>[4x]MQRVVVAIVAKRVDGEFMVFTHSGKKNTGILLRDWVVEVEKRGAGEILLTSIDRVGTKSGYDTEMIRFVRPLTTLPIIASGGAGKMEHFLEAFLAGADKVSINTAAVENPSLITQIAQTFGSQAVVVAIVAKRVDGEFMVFTHSGKKNTGIL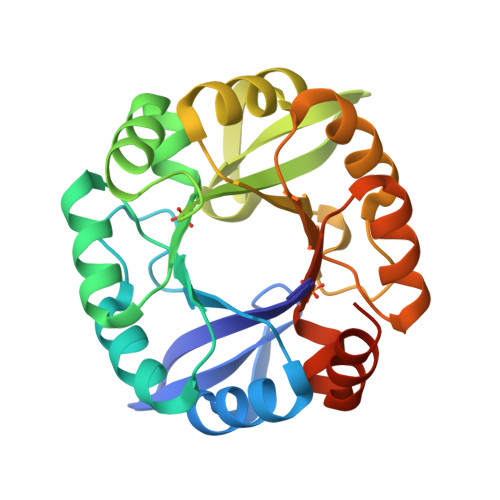LRDWVVEVEKRGAGEILLTSIDRVGTKSGYDTEMIRFVRPLTTLPIIASGGAGKMEHFLEAFLAGADKVSINTAAVENPSLITQIAQTFGSLEHHHHHH>MSVRLVLAKGREKSLLRRHPWVFSGAVARMEGKASLGETIDIVDHQGKWLARGAYSPASQIRARVWTFDPSESIDIAFFSRRLQQAQKWRDWLAQKDGLDSYRLIAGESDGLPGITIDRFGNFLVLQLLSAGAEYQRAALISALQTLYPECSIYDRSDVAVRKKEGMELTQGPVTGELPPALLPIEEHGMKLLVDIQHGHKTGYYLDQRDSRLATRRYVENKRVLNCFSYTGGFAVSALMGGCSQVVSVDTSQEAL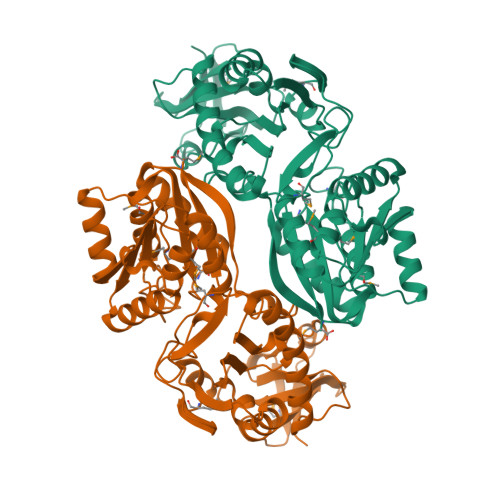DIARQNVELNKLDLSKAEFVRDDVFKLLRTYRDRGEKFDVIVMDPPKFVENKSQLMGACRGYKDINMLAIQLLNEGGILLTFSCSGLMTSDLFQKIIADAAIDAGRDVQFIEQFRQAADHPVIATYPEGLYLKGFACRVM[2x]> MQIFRDVSKLLVERVDPKILNLFRLLGKFGDEVNMPVYVVGGFVRDLLLGIKNLDIDIVVEGNALEFAEYAKRFLPGKLVKHDKFMTASLFLKGGLRIDIATARLEYYESPAKLPDVEMSTIKKDLYRRDFTINAMAIKLNPKDFGLLIDFFGGYRDLKEGVIRVLHTLSFVDDPTRILRAIRFEQRFDFRIEETTERLLKQAVEEGYLERTTGPRLRQELEKILEEKNPLKSIRRMAQFDVIKHLFPKTYYTPSMDEKMENLFRNIPWVEENFGEVDRFYAVLHVFLEFYDDESWKEVRDRYSLRRNLINEIRHVEKSAPALLEMLSERVPASFVYPLVKGVSNETICHFLAYLSGEKEGLFKSYLLKIKNTKLEKINGEYLIRKGITSGKIIGEVLEKILMKKLDGDTRDEEEILEEVLASLETEGKLAAALE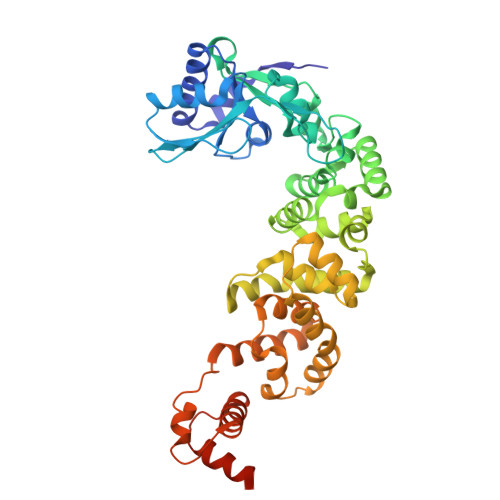HHHHHH Fluorescent proteins have facilitated major breakthroughs in modern molecular cell biology. They are widely used for studying biological events, such as cellular trafficking and endocytosis, and have contributed to the development of innovations such as multiphoton microscopy, genetically-encoded sensors, and super-resolution microscopy. mKate, a derivative of eqFP578 from Entacmaea quadricolor, is a bright, monomeric, far-red fluorescent protein with excitation and emission peaks at 588 nm and 635 nm, respectively. Structural characterization of mKate under different conditions revealed the pH-dependent trans-cis isomerization of its chromophore, a discovery that further aided the development of mKate variants with enhanced optical properties. Using a structure-informed approach, we introduced a minimal set of two mutations in the chromophore environment of mKate. The first mutation, S158A, has been shown to destabilize the trans conformation of the chromophore, whereas the second mutation, S143C, was intended to impact the cis conformation.

In contrast, the single-mutant variant mKateS158A, which lacks the S143C mutation, has predominately one absorbance peak at 588 nm and emits strongly at 633 nm, giving the protein a visible red color. Mutation S158A disrupts the hydrogen bond that stabilizes the trans-conformation and as a result the chromophore populates the cis-conformation in the mKate variants at physiological pH. As predicted, the chromophore of mKateS158A at pH 7.0 exists entirely in its cis-conformation. The phenolate forms hydrogen bonds with S143 and a water molecule (Wat1), as observed in the structure of mKate at neutral pH. In contrast to mKate structures, residues R197, E215 and several chromophore-coordinating water molecules undergo major structural rearrangements in mKateS158A. R197 adopts a different rotamer conformation and forms hydrogen bonds with E215 and E145, while in mKate, R197 forms a hydrogen bond with S143 and S158. Changes in the hydrogen bond network reveal a cavity in mKateS158A (and GmKate) that is filled by a water molecule (Wat3). The particular conformation of R197 in mKateS158A positions its guanidine group above the conjugated bond between the Y62 phenol ring and the imidazole moiety, presumably altering the conjugated π electron density distribution on the chromophore via a cation-π interaction, as has been proposed for mNeptune. The crystal structure of mKateS158A reveals three potential proton wires. In pathway A, the phenolic oxygen is in direct contact with the side chain of S143, which is hydrogen-bonded to R197 through a water-mediated interaction.

>AAASMSALITENMHMKLYMEGTVNNHHFKCTSEGEGKPYEGTQTMRIKVVEGGPLPFAFDILATSFMYGSKTFINHTQGIPDFFKQSFPEGFTWERVTTYEDGGVLTATQDTSLQDGCLIYNVKIRGVNFPSNGPVMQKKTLGWEASTEMLYPADGGLEGRADMALKLVGGGHLICNLKTTYRSKKPAKNLKMPGVYYVDRRLERIKEADKETYVEQHEVAVARYCDLPSKLAHK[4x]> KPEPTDEEWELIKTVTEAHVATNAQGSHWKQKRKFLPEDIGQAPIVNAPEGGKDDLEAFSHFTKIITPAITRVVDFAKKLPMFCELPCEDQIILLKGCCMEIMSLRAAVRYDPESETLTLNGEMAVTRGQLKNGGLGVVSDAIFDLGMSLSSFNLDDTEVALLQAVLLMSSDRPGLACVERIEKYQDSFLLAFEHYINYRKHHVTHFWPKLLMKVTDLRMIGACHASRFLHMKVECPTELFPPLFLEVFE;> ENALLRYLLDK

The thyroid hormone receptors (THRs) are nuclear hormone receptors regulated by endogenous thyroid hormones, including the inactive prohormone thyroxine (T4) and the bioactive hormone 3,3′,5-triiodothyronine (T3), which are critical for development regulation and metabolic homeostasis. As ligand-regulated nuclear receptors, THRs have a structurally conserved LBD that allows the binding of distinct ligands (Burris et al., 2013). Following the ligand binding, the function of THRs is mediated through the selective recruitment or release of specific coregulators, like the family of steroid receptor coactivators (SRCs) (Li et al., 2003, Jin and Li, 2010, Savkur and Burris, 2004), as a heterodimeric complex with retinoid X receptor (RXR) (Putcha et al., 2012, Kojetin et al., 2015, Mangelsdorf and Evans, 1995). Although the defects in any of the processes in thyroid hormone transport and synthesis can all contribute to RTH, in most cases the disorder involves defective thyroid hormone receptors, resulting in reduced T3 binding and disruptive thyroid hormone signaling.

As expected, the native ligand T3 abolished or substantially diminished the transcriptional activity of four THRβ mutants associated with thyroid hormone resistance, V264D, H435L, R438H, and R438W, respectively (Wakasaki et al., 2016, Nomura et al., 1996, Sabet and Pallotta, 2011, Narumi et al., 2010). Surprisingly, the treatment of roxadustat either enhanced or retained the transcriptional activity of these THRβ mutants, all leading to higher induced transcriptional activity than those of T3. In contrast, the binding of roxadustat resulted in higher Tm values for four TRβ mutants than that of T3. Although all four mutant residues are located in the THRβ LBD, H435 is the only one that directly contacts ligands T3 or roxadustat, whereas the rest of the mutant residues are located outside the ligand-binding pocket, not in the range to form intimate contacts with the ligands, which makes us wonder how these mutants influence the ligand binding. To unravel the molecular basis for the RTH of the THRβ mutants and further their beneficial susceptibility to roxadustat, we performed structural studies on the THRβ mutants complexed with roxadustat. The structural analysis further revealed an apparent conformational change of residue H435 on helix 10 of THRβ for all four mutants, resulting in the loss of a critical hydrogen bond between THRβ and a critical hydroxy group of T3, which is also conserved for the other THR ligands identified so far, explaining the severely reduced THRβ activity by T3. Specifically, in addition to the direct mutation of H435 to the hydrophobic leucine of THRβ H435L, the allosteric conformational changes of THRβ H435 were coupled with several intermediate structural changes, predominantly in helix 10, which were initiated by mutants R438H, R438W, or V264D, consequently leading to impaired T3 binding.> IIGGTECKPHSRPYMAYLEIVTSNGPSKFCGGFLIRRNFVLTAAHCAGRSITVTLGAHNITEEEDTWQKLEVIKQFRHPKYNTSTLHHDIMLLKLKEKASLTLAVGTLPFPSQKNFVPPGRMCRVAGWGRTGVLKPGSDTLQE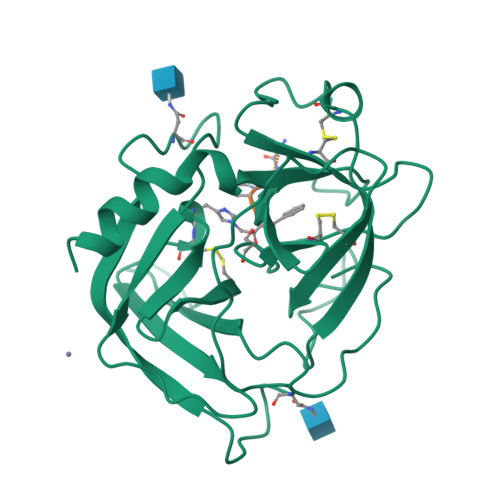VKLRLMDPQACSHFRDFDHNLQLCVGNPRKTKSAFKGDSGGPLLCAGAAQGIVSYGRSDAKPPAVFTRISHYQPWINQILQAN;> AAPFX>[2x]GLFDI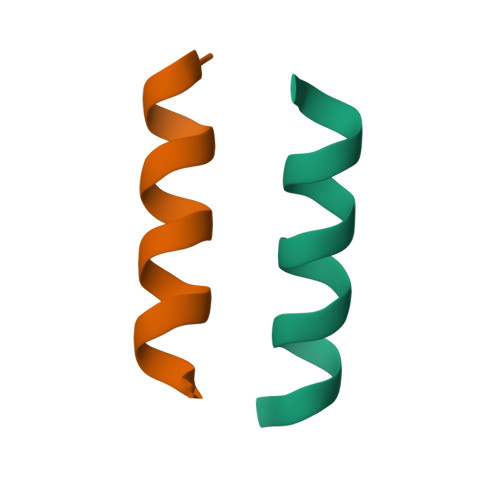IKKVASVIGGL>AGAGAMYDIKKWRHIFKLDPAKHISDDDLDAICMSQTDAIMIGGTDDVTEDNVIHLMSKIRRYPLPLVLEISNIESVMPGFDFYFVPTVLNSTDVAFHNGTLLEALKTYGHSIDFEEVIFEGYVVCNADSKVAK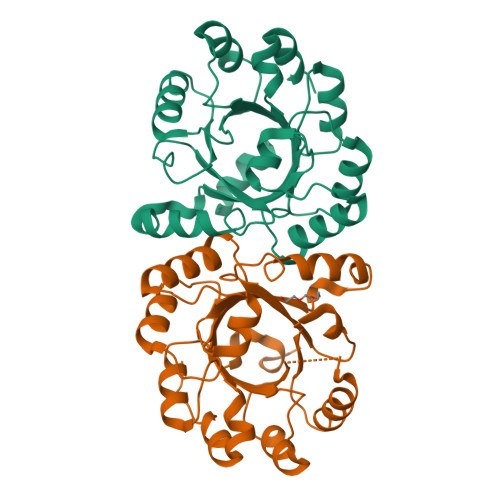HTKANTDLTTEDLEAYAQMVNHMYRLPVMYIEYSGIYGDVSKVQAVSEHLTETQLFYGGGISSEQQATEMAAIADTIIVGDIIYKDIKKALKTVKIKESSK[2x]> SVRSSSRTPSDKPVAHVVANPQAEGQLQWLNRRANALLANGVELRDNQLVVPSEGLYLIYSQVLFKGQGCPSTHVLLCHTISRIAVSYQTKVNLLSAIKSPCQRETPEGAEAKPWYEPIY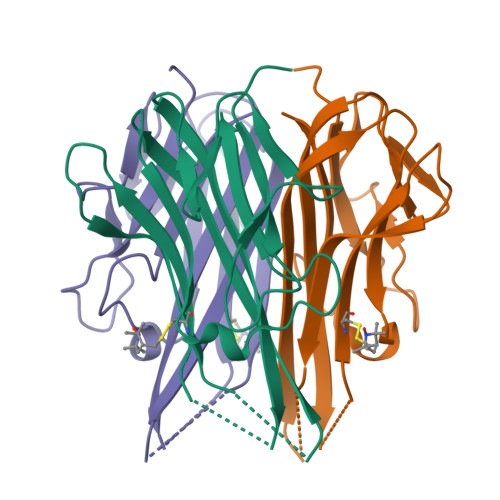LGGVFQLEKGDRLSAEINRPDYLDFAESGQVYFGIIAL The tripartite signalling system YfiBNR in P. aeruginosa modulates intracellular c-di-GMP levels in response to signals received in the periplasm and is a key regulator of the SCV phenotype. The effector protein YfiN (also known as TpbB or PA1120) is an integral inner membrane protein that functions as a diguanylate cyclase, consisting of a periplasmic PAS domain, a cytoplasmic HAMP domain and a catalytic GGDEF domain. The third component of the YfiBNR signalling system, YfiR, has a key role in the signal transduction process by bridging YfiN in the inner membrane and YfiB in the outer membrane. YfiB can release the repression of YfiN by sequestering YfiR at the outer membrane, which requires both membrane anchoring and peptidoglycan binding by YfiB for full activity.

However, only YfiB(59–168) could be crystallized in a complex with a C71S mutant of YfiR; attempts to co-crystallize YfiB(27–168) with wild-type YfiR yielded poorly diffracting crystals. The resulting structure to 1.97 Å resolution reveals one YfiR monomer binds to one monomer of YfiB(59–168). The interface area of the complex is 1,053 Å2, with YfiB burying 1,024 Å2 (16% of the total accessible surface area) and YfiR burying 1,079 Å2 (13% of the total accessible surface area). YfiR interacts with YfiB exclusively through its C-terminal region. Strand β1 of YfiB is completely unwound, allowing strand β7 of YfiR to stack against strand β4 of YfiB in an anti-parallel manner to form an extended β-sheet spanning both proteins. Furthermore, both Glu163 and Ile169 of YfiR, which have previously been shown to interact with YfiN24, also interact with residues in YfiB, suggesting that YfiR uses this same region to bind to both YfiN in the inner membrane and YfiB in the outer membrane. The extensive interface between YfiB and YfiR includes a number of hydrogen bonds and salt bridges: Arg96 of YfiB forms a hydrogen bond with Glu144 of YfiR and a salt bridge with Glu163. Met59 of YfiB inserts into this hydrophobic pocket and interacts with the lining residues such that its side chain is 5.3 Å from Phe151. The choice of a C71S mutant of YfiR breaks the Cys71-Cys110 disulfide bond, but the Cys145-Cys152 disulfide bond remains intact in the C-terminal of the protein upon binding to YfiB. In this arrangement, YfiB binds to each end of the YfiR dimer such that the N-terminal linkers are situated at one side of the complex and the conserved PG-binding sites are located on the opposing side.

> MPSLPTLQPLDLYRRTLACLVLAVSCLGGGGLWADDARTSIEQRSNAVSQVLLGIFSYVRWPKEPAVLQLSVVGPTEYADGLLRGMVQANGRRVHAERRAVDNPDLGTLCNVIYLGVVDERERQQVFRSLAGHPVLSISERGTECSVGSMFCLNVGGPRITFEANLDSIARSGVRVHPSVLKLARRQATP;> MLPQRLHPSRLLALALFSLVLGLAGCQTKPPQTGLSAEQIAVLQEQGFELRDEGWPGSMSSKVLFGNNLDRLNPDSRNTLTKIARALLAVDIDKVRLEGHTDNYGDEGYNQKLSERRAESVAAVFREAGMPAANIEVRGLGMSKPVADNKTRAGRSENRRVAIIVPAE> SMSNFVNLDIFSNYQKYIDNEQEVRENIRIVVREIEHLSKEAQIKLQIIHSDLSQISAACGLARKQVELCAQKYQKLAELVPAGQYYRYSDHWTFITQRLIFIIALVIYLEAGFLVTRETVAEMLGLKISQ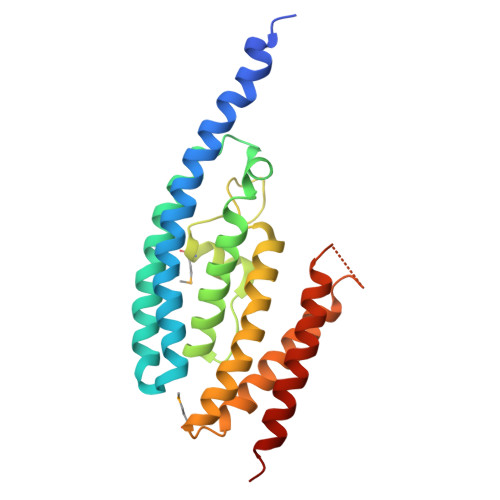SEGFHLDVEDYLLGILQLASELSRFATNSVTMGDYERPLNISHFIGDLNTGFRLLNLKNDGLRKRFDALKYDVKKIEEVVYDVSIRG>[4x]MASVQLQNVTKAWGEVVVSKDINLDIHEGEFVVFVGPSGCGKSTLLRMIAGLETITSGDLFIGEKRMNDTPPAERGVGMVFQSYALYPHLSVAENMSFGLKLAGAKKEVINQRVNQVAEVLQLAHLLDRKPKALSGGQRQRVAIGRTLVAEPSVFLLDEPLSNLDAALRVQMRIEISRLHKRLGRTMIYVTHDQVEAMTLADKIVVLDAGRVAQVGKPLELYHYPADRFVAGFIGSPKMNFLPVKVTATAIDQVQVELPMPNRQQVWLPVESRDVQVGANMSLGIRPEHLLPSDIADVILEGEVQVVEQLGNETQIHIQIPSIRQNLVYRQNDVVLVEEGATFAIGLPPERCHLFREDGTACRRLHKEPGVASASHHHHHH;>[2x]MAQGEYLFAITTLILSSAGLYIFANRKAYAWRYVYPGMAGMGLFVLFPLVCTIAIAFTNYSSTNQLTFERAQEVLLDRSWQAGKTYNFGLYPAGDEWQLALSDGETGKNYLSDAFKFGGEQKLQLKETTAQPEGERANLRVITQNRQALSDITAILPDGNKVMMSSLRQFSGTQPLYTLDGDGTLTNNQSGVKYRPNNQIGFYQSITADGNWGDEKLSPGYTVTTGWKNFTRVFTDEGIQKPFLAIFVWTVVFSLITVFLTVAVGMVLACLVQWEALRGKAVYRVLLILPYA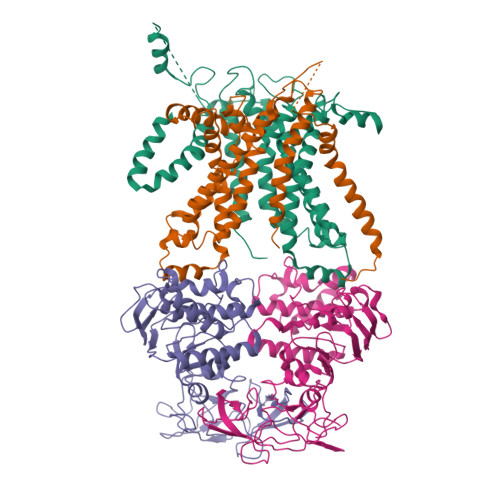VPSFISILIFKGLFNQSFGEINMMLSALFGVKPAWFSDPTTARTMLIIVNTWLGYPYMMILCMGLLKAIPDDLYEASAMDGAGPFQNFFKITLPLLIKPLTPLMIASFAFNFNNFVLIQLLTNGGPDRLGTTTPAGYTDLLVNYTYRIAFEGGGGQDFGLAAAIATLIFLLVGALAIVNLKATRMKFD;>[2x]MAMVQPKSQKARLFITHLLLLLFIAAIMFPLLMVVAISLRQGNFATGSLIPEQISWDHWKLALGFSVEQADGRITPPPFPVLLWLWNSVKVAGISAIGIVALSTTCAYAFARMRFPGKATLLKGMLIFQMFPAVLSLVALYALFDRLGEYIPFIGLNTHGGVIFAYLGGIALHVWTIKGYFETIDSSLEEAAALDGATPWQAFRLVLLPLSVPILAVVFILSFIAAITEVPVASLLLRDVNSYTLAVGMQQYLNPQNYLWGDFAAAAVMSALPITIVFLLAQRWLVNGLTAGGVKG>[2x]MKRKIIYLASPYGFSQQQKTLLLPPIVRALEALGIEVWEPFARNNQIDFSQADWAYRVAQANLQDVKNCDGIFAVVNG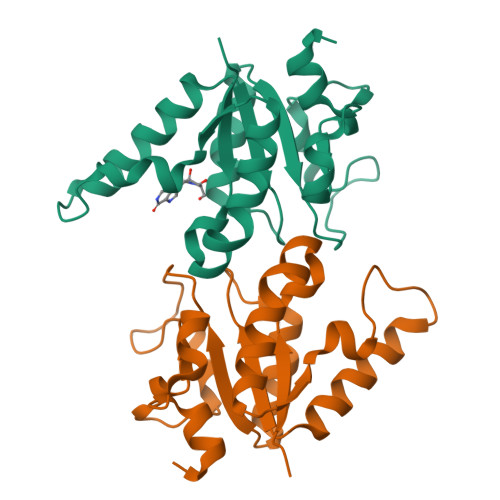TPPDEGVMVELGMAIALNKAIFLFRDDFRRCSDNERYPLNLMLFAGLPEIGWENYYYTSVDEIQSHDKALYKWLTGM>ADNYAATRYPIILVHGLTGTDKYAGVLEYWYGIQEDLQQRGATVYVANLSGFQSDDGPNGRGEQLLAYVKTVLAATGATKVNLVGHSQGGLTSRYVAAVAPDLVASVTTIGTPHRGSEFADFVQGVLAYDPTGLSSTVIAAFVNVFGILTSSSNNTNQDALAALKTLTTAQAATYNQNYPSAGLGAPGSCQTGAPTETVGGNTHLLYSWAGTAIQPTIS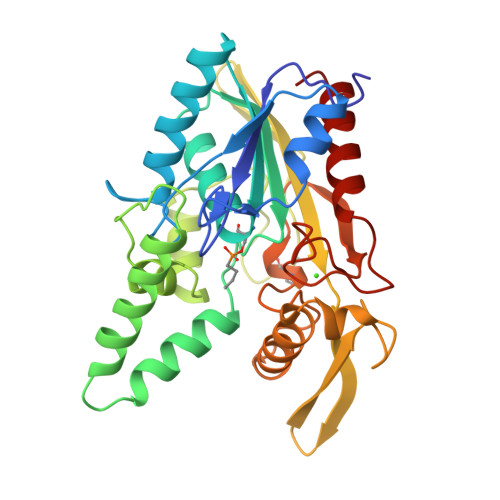VFGVTGATDTSTIPLVDPANALDPSTLALFGTGTVMVNRGSGQNDGVVSKCSALYGQVLSTSYKWNHLDEINQLLGVRGANAEDPVAVIRTHANRLKLAGV[2x]>MDDTPHFRIGVAQCSDDSWRHKMNDEILREAMFYNGVSVEIRSAGDDNSKQAEDVHYFMDEGVDLLIISANEAAPMTPIVEEAYQKGIPVILVDRKILSDKYTAYIGADNYEIGRSVGNYIASSLKGKGNIVELTGLSGSTPAMERHQGFMAAISKFPDIKLIDKADAAWERGPAEIEMDSMLRRHPKIDAVYAHNDRIAPGAYQAAKMAGREKEMIFVGIDALPGKGNGLELVLDSVLDATFIYPTNGDKVLQLAMDILEKKPYPKETVMNTAVVDRTNAHVMQLQTTHISELDKKIETLNGRIGGYLSQVATQQ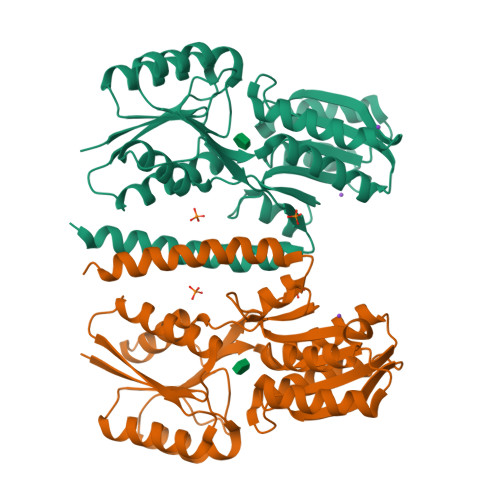VLEHHHHHH[2x]>PKFPRVKNWEVGSITYDTLSAQAQQDGPCTPRRCLGSLVFPRKLQGRPSPGPPAPEQLLSQARDFINQYYSSIKRSGSQAHEQRLQEVEAEVAATGTYQLRESELVFGAKQAWRNAPRCVGRIQWGKLQVFDARDCRSAQEMFTYICNHIKYATNRGNLRSAITVFPQRCPGRGDFRIWNSQLVRYAGYRQQDGSVRGDPANVEITELCIQHGWTPGNGRFDVLPLLLQAPDEPPELFLLPPELVLEVPLEHPTLEWFAALGLRWYALPAVSNMLLEIGGLEFPAAPFSGWYMSTEIGTRN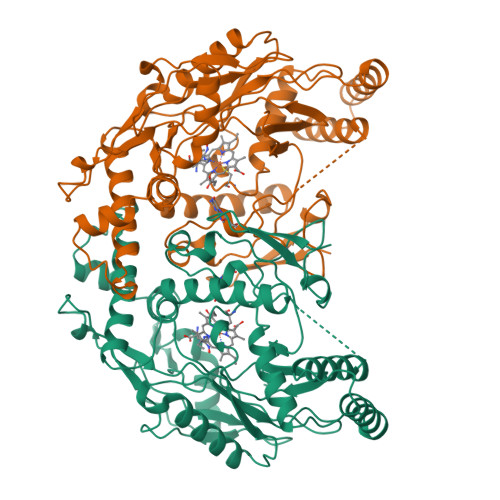LCDPHRYNILEDVAVCMDLDTRTTSSLWKDKAAVEINVAVLHSYQLAKVTIVDHHAATASFMKHLENEQKARGGCPADWAWIVPPISGSLTPVFHQEMVNYFLSPAFRYQPDPWKGSAAKGTGITR[2x]>MHHHHHHLEGSALPSTFVAEKWENFKTTYARSYVNAKEETFRKQIFQKKLETFEEHNEKYRQGLVSYTLGVNLFTDMTPEEMKAYTHGLIMPADLHKNGIPIKTREDLGLNASVRYPASFDWRDQGMVSPVKNQGSCGSSWAFSSTGAIESQMKIANGAGYDSSVSEQQLVDCVPNALGCSGGWMNDAFTYVAQNGGIDSEGAYPYEMADGNCHYDPNQVAARLSGYVYLSGPDENMLADMVATKGPVAVAFDADDPFGSYSGGVYYNPT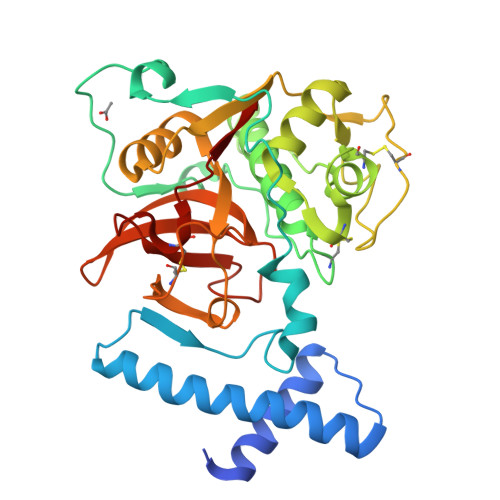CETNKFTHAVLIVGYGNENGQDYWLVKNSWGDGWGLDGYFKIARNANNHCGIAGVASVPTL[2x]>[20x]EFDRADILYNIRQTSRPDVIPTQRDRPVAVSVSLKFINILEVNEITNEVDVVFWQQTTWSDRTLAWNSSHSPDQVSVPISSLWVPD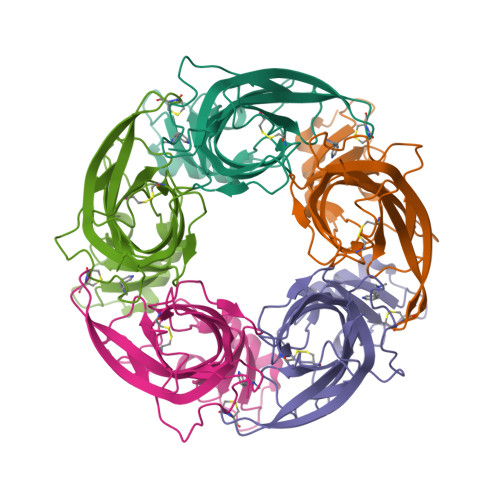LAAYNAISKPEVLTPQLARVVSDGEVLYMPSIRQRFSCDVSGVDTESGATCRIKIGSWTHHSREISVDPTTENSDDSEYFSQYSRFEILDVTQKKNSVTYSCCPEAYEDVEVSLNFRKKGRSEIL> MNLPTAQEVQGLMARFIELVDVGDIEAIVQMYADDATVEDPFGQPPI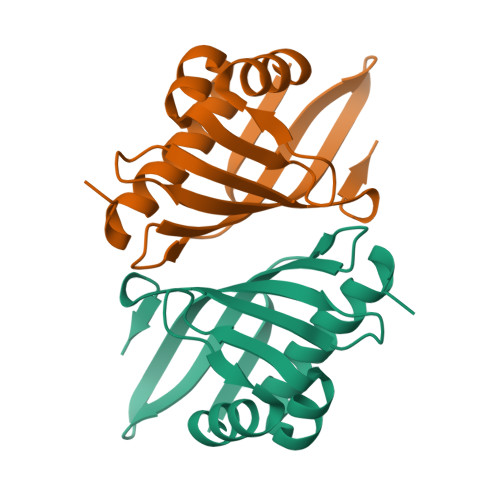HGREQIAAFFRQGLGGGKVRACLTGPVRASHNGCGAMPFRVEMVWNGQPCALDVIDVMRFDEHGRIQTMQAYWSEVNLSVREPQ>[5x]GQDMVSPPPPIADEPLTVNTGIYLIECYSLDDKAETFKVNAFLSLSWKDRRLAFDPVRSGVRVKTYEPEAIWIPEIRFVNVQNARDADVVDISVSPDGTVQYLERFSARVLSPLDFRRYPFDSQTLHIYLIVRSVDTRNIVLAVDLEKVGKNDDVFLTGWDIESFTAVVKPANFALEDRLESKLDYQLRISRQYFSYIPNIILPMLFILFISWTAFWSTSYEANVTLVVSTLIAHIAFNILVETNLPKTPYMTYTGAIIFMIYLFYFVAVIEVTVQHYLKVESQPARAASITRASRIAFPVVFLLANIILAFLFFGF

At present, the best structurally characterized pLGIC is the G. violaceus ligand-gated ion channel (GLIC), of prokaryotic origin. Each subunit consists of an extracellular domain (ECD), predominantly in a β-sandwich fold, and a transmembrane domain (TMD) composed of four helices, labeled M1–M4. However, the GLIC is a pH-gated channel, activated by lowering the pH, with a maximal activation at pH 4 and a pH50 around 5. We instead found that proton activation is a complex multiple loci mechanism, with the key contribution stemming from the coupling interface between the extracellular and transmembrane domain, with E35 acting as a key proton-sensing residue.

In the lower part of the ECD, the principal (+) face also carries two acidic residues, E82 and D115. E82Q and D115N display significantly higher proton sensitivity than E82A and D115A, respectively. Assuming that Gln and Asn faithfully mimic protonated side chains of Glu and Asp, this would suggest that residues E82 and D115 are also proton sensors. To investigate this idea, the structures of E82Q and E82A were solved at pH 4. The E82A structure is similar to that of the Wt pH 4 structure, whereas that of E82Q shows a marked local reorganization of the Q82 moiety. Assuming E82 to be in a protonated state at pH 4, Gln is not a good mimic of a protonated Glu residue because Q82 is engaged in a completely different set of interactions with neighboring residues. Therefore, the E82Q mutant phenotype is likely due to local side chain reorganizations of Y28 and F156 rather than being a proton sensor itself. There are no significant differences, measured as 5-fold over Wt, seen in the backbone Cα residues of any of the resolved structures, with the exception of E35A and E82Q. The E82Q side chain takes on a different rotamer, causing a local change in the backbone, as well as a cascading rotamer/conformational change in Y28 and F156, the latter of which flips out towards the aqueous environment. All structures were in the apparently open conformation.> SMEELSQALASSFSVSQDLNSTAAPHPRLSQYKSKYSSLEQSERRRRLLELQKSKRLDYVNHARRLAEDDWTGMESEEENKKDDEEMDIDTVKKLPKHYANQLMLSEWLIDVPSDLGQEWIVVVCPVGKRALIVASRGSTSAYTKSGYCVNRFSSLLPGGNRRNSTAKDYTILDCIYNEVNQTYYVLDVMCWRGHPFYDCQTDFRFYWMHSKLPEEEGLGEKTKLNPFKFVGLKNFPCTPESLCDVLSMDFPFEVDGLLFYHKQTHYSPGSTPLVGWLRPYMVSDVLGVAVPAGPLTTKPDYAGHQLQQIMEHKKSQKEGMKE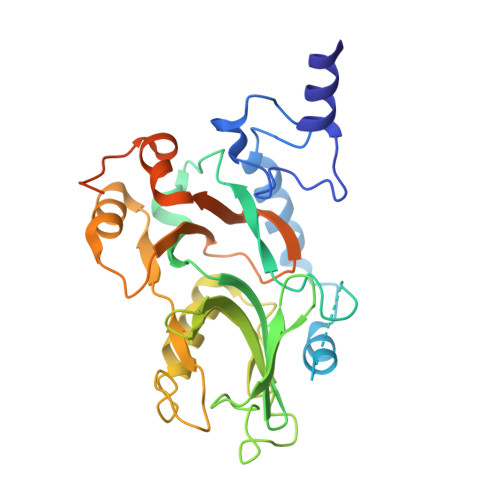KLTHKA>MEAPAAVVTGAAKRIGRAIAVKLHQTGYRVVIHYHNSAEAAVSLADELNKERSNTAVVCQADLTNSNVLPASCEEIINSCFRAFGRCDVLVNNASAFYPTPLVQGDHEDNSNGKTVETQVAELIGTNAIAPFLLTMSFAQRQKGTNPNCTSSNLSIVNLCDAMVDQPCMAFSLYNMGKHALVGLTQSAALELAPYGIRVNGVAPGVSLLPVAMGEEEKDKWRRKVPLGRREASAEQIADAVIFLVSGSAQYITGSIIKVDGGLSLVHA[4x]

The protozoan Trypanosoma brucei has a functional pteridine reductase (TbPTR1), an NADPH-dependent short-chain reductase that participates in the salvage of pterins, which are essential for parasite growth. PTR1 displays broad-spectrum activity with pterins and folates, provides a metabolic bypass for inhibition of the trypanosomatid dihydrofolate reductase and therefore compromises the use of antifolates for treatment of trypanosomiasis. PTR1 is a short-chain dehydrogenase/reductase (SDR) able to catalyse the NADPH-dependent two-stage reduction of oxidized pterins to the active tetrahydro-forms. The TbPTR1 subunit forms a single α/β-domain constructed around a seven-stranded parallel β-sheet sandwiched between two sets of α-helices.

Catalytic properties of recombinant TbPTR1 and inhibition by the archetypal antifolate methotrexate have been characterized and the crystal structure of the ternary complex with cofactor NADP+ and the inhibitor determined at 2.2 Å resolution. The asymmetric unit consists of a homotetramer, which represents the functional unit, and overlays of the 251 residues common to each of the four subunits show a root mean square deviation (r.m.s.d.) range in Cα positions of 0.19–0.31 Å (mean 0.25 Å). The functional tetramer displays point group 222, with two active sites, separated by approximately 25 Å, on each side of the assembly. The association between TbPTR1/NADP+ and MTX is primarily through interactions with the pteridine moiety, which is sandwiched between the nicotinamide and Phe97. Four of the six N atoms of the pteridine moiety make direct interactions: N1 with the α-phosphate group of the cofactor and is likely protonated, N2 donates hydrogen bonds to the side-chain hydroxyl and main-chain carbonyl groups of Ser95, N3 accepts a hydrogen bond from the 2′ hydroxyl group of the nicotinamide ribose. The para-aminobenzoic acid (pABA) and γ-Glu components of MTX are directed out of the binding site with the γ-Glu tail of MTX directed towards the N-terminus of the β6-α6 loop. The presence of the larger tryptophan side-chain at this position in TbPTR1 compared with a histidine in LmPTR1, or tyrosine in both TcPTR2 and LtPTR1 in conjunction with the α6 adjustment reduces the size of the pABA binding region in the enzyme derived from the African trypanosome and introduces a significant chemical change in this area of the active site. In TbPTR1 the C-terminal basic residue is His267 but the presence of Trp221 in conjunction with a chemically modified Cys168 (the corresponding residue is Leu184 in LmPTR1) occludes the presence of a solvent network in this part of the active site. The modification of Cys168 by reaction with cacodylate buffer to form dimethylarsinoyl cysteine is intriguing but not unusual in protein chemistry and it is uncertain whether such reactivity has a biological function in T. brucei.> SEALQQEIAKIDEEIQKCIRDKEAVDAFLPAHGEQLAAIPTDVNFVT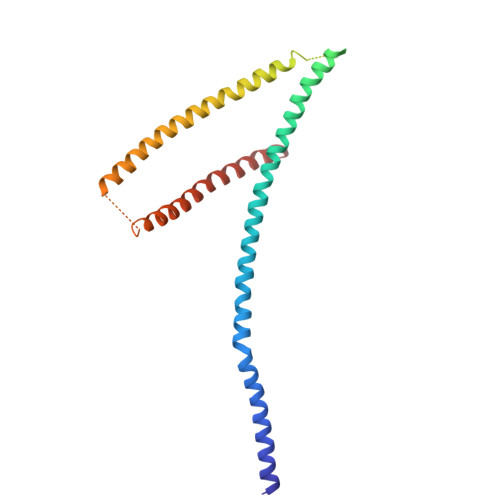RKSEGAHNALSSDILAIDQLRELVKQDADNARLSFKAIDNLKLPMQYHQAGLWSKQMGGAGTAGASGASADADGQSNADLISYFSKTADEMEEMMKKFEKTITEIEAHLTGVEAHAMAMQNVAAQSRNAAQGGVDERVYELAAVLREFEESILKVAGVVGGVKEGVTELQLRDFM>SNANALVEDFERELGRMLSPFELEDLQKTVSD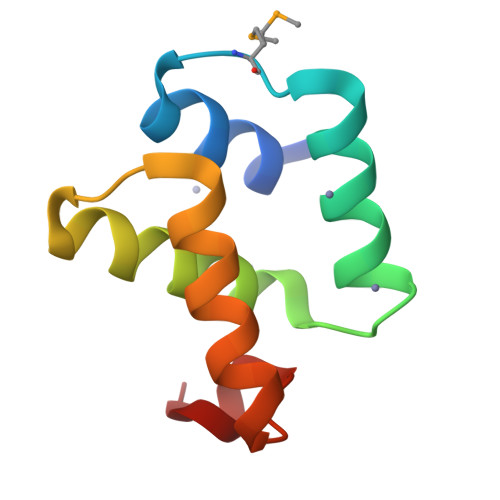DKTDPDLVRSALREAVFNGKTNWNYIQAILRNWRHEGISTLRQVEE[2x]> VRPLNCIVAVSQNMGIGKNGDRPWPPLRNEFKYFQRMTTTSSVEGKQNLVIMGRKTWFSIPEKNRPLKDRINIVLSRELKEPPRGAHFLAKSLDDALRLIEQPELASKVDMVWIVGGSSVYQEAMNQPGHLRLFVTRIMQEFESDTFFPEIDLGKYKLLPEYPGVLSEV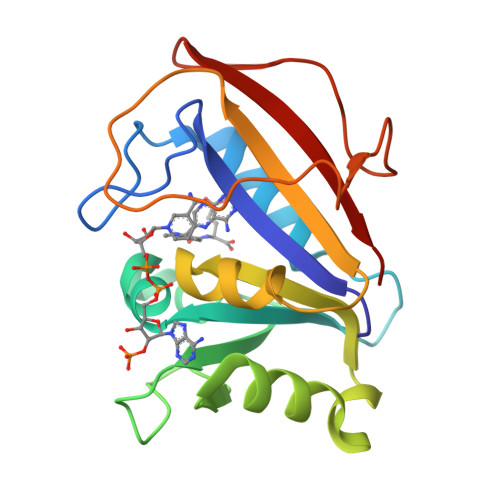QEEKGIKYKFEVYEKKD>MALQNEKNSRYLLRDWKPENPAFWENKGKHIARRNLWISVSCLLLAFCVWMLFSAVTVNLNKIGFNFTTDQLFLLTALPSVSGALLRVPYSFMVPIFGGRRWTVFSTAILIIPCVWLGIAVQNPNTPFGIFIVIALLCGFAGANFASSMGNISFFFPKAKQGSALGINGGLGNLGVSVMQLVAPLVIFVPVFAFLGVNGVPQADGSVMSLANAAWIWVPLLAIATIAAWSGMNDIASSRASIADQLPVLQRLHLWLLSLLYLATF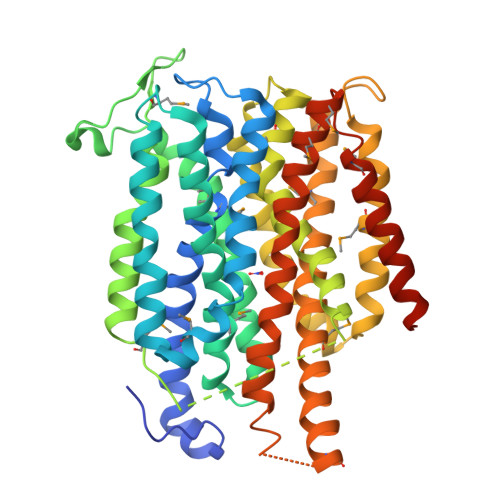GSFIGFSAGFAMLAKTQFPDVNILRLAFFGPFIGAIARSVGGAISDKFGGVRVTLINFIFMAIFSALLFLTLPGTGSGNFIAFYAVFMGLFLTAGLGSGSTFQMIAVIFRQITIYRVKMKGGSDEQAHKEAVTETAAALGFISAIGAVGGFFIPQAFGMSLNMTGSPVGAMKVFLIFYIVCVLLTWLVYGRRKFSQKLEVLFQ[2x]>[2x]EAKLAKYEADLAKYKKEFAAYTAALAEAESKKKQDGYLSEPRSQSLNFKSEPNAIRTIDSSVHQYGQQELDALVKSWGISPTNPDRKKSRAYSYFNAINSNNTYAKLVLEKDKPVDVTYTGLKNSSFNGKKISKVVYT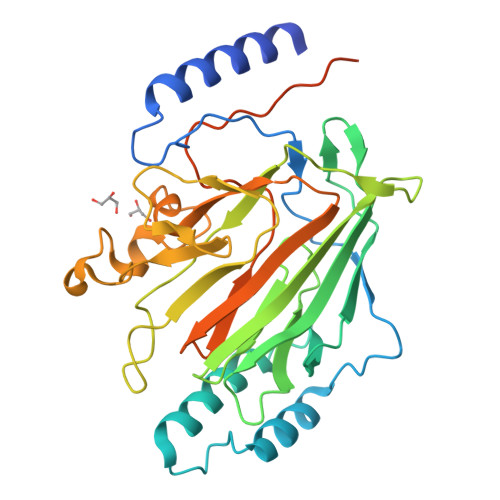YTLKETGFNDGTKMTMFASSDPTVTAWYNDYFTSTNINVKVKFYDEEGQLMNLTGGLVNFSSLNRGNGSGAIDKDAIESVRNFNGRYIPISGSSIKIHENNSAYADSSNAEKSLGARWNTSEWDTTSSPNNWYGAIVGEITQSEISFNMASSKSGNIWFAFNSNINAIGVPTKPVAPTAPTQPMYETEKPLEPAPVAPSYENEPTPPVKTP>[2x]MKSKKILIVGAGFSGAVIGRQLAEKGHQVHIIDQRDHIGGNSYDARDSETNVMVHVYGPHIFHTDNETVWNYINKHAEMMPYVNRVKATVNGQVFSLPINLHT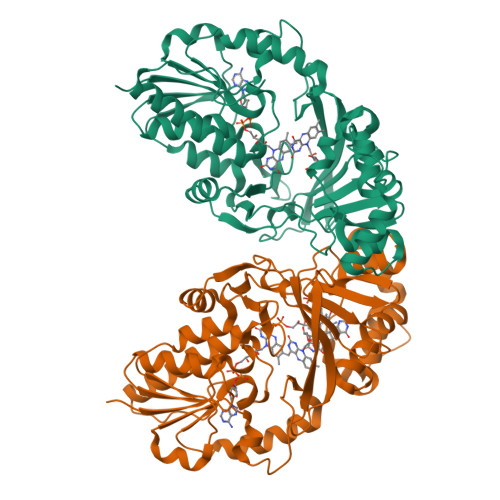INQFFSKTCSPDEARALIAEKGDSTIADPQTFEEQALRFIGKELYEAFFKGYTIKQWGMQPSELPASILKRLPVRFNYDDNYFNHKFQGMPKCGYTQMIKSILNHENIKVDLQREFIVDERTHYDHVFYSGPLDAFYGYQYGRLGYRTLDFKKFIYQGDYQGCAVMNYCSVDVPYTRITEHKYFSPWEQHDGSVCYKEYSRACEENDIPYYPIRQMGEMALLEKYLSLAENETNITFVGRLGTYRYLDMDVTIAEALKTAEVYLNSLTDNQPMPVFTVSVGHHHHHH> HMERPESELIRQSWRVVSRSPLEHGTVLFARLFALEPSLLPLFQGGGQFSSPEDSLSSPEFLDHIRKVMLVIDAAVTNVEDLSSLEEYLTS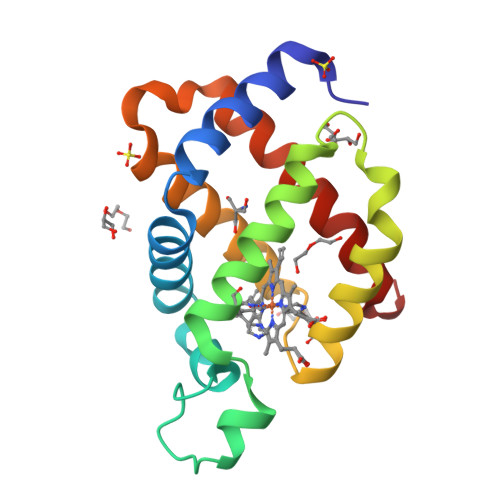LGRKHRAVGVRLSSFSTVGESLLYMLEKSLGPDFTPATRTAWSRLYGAVVQAMSRGWDG>MGESERSEAFGIPRDSPLSSGDAAELEQLRREAAVLREQLENAVGSHAPTRSARDIHQLEARIDSLAARNSKLMETLKEARQQLLALREEVDRLGQPPSGYGVLLATHDDDTVDVFTSGRKMRLTCSPNIDAASLKKGQTVRLNEALTVVEAGTFEAVGEISTLREILADGHRALVVGHADEERVVWLADPLIAEDLPDGLPEALNDDTRPRKLRPGDSLLVDTKAGYAFERIPKAEVEDLVLEEVPDVSYADIGGLSRQIEQIRDAVELPFLHKELYREYSLRPPKGVLLYGPPGCGKTLIAKAVANSLAKKMAEVRGDDAHEAKSYFLNIKGPELLNKFVG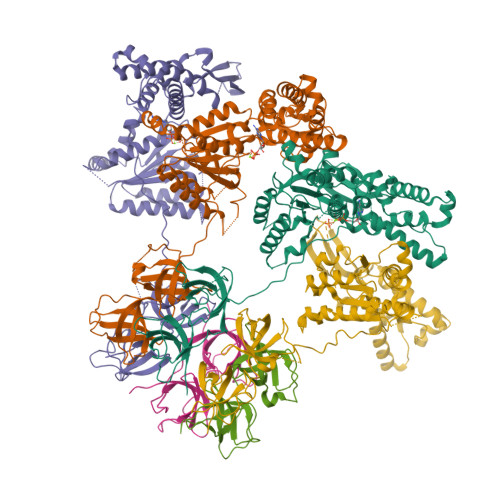ETERHIRLIFQRAREKASEGTPVIVFFDEMDSIFRTRGTGVSSDVETTVVPQLLSEIDGVEGLENVIVIGASNREDMIDPAILRPGRLDVKIKIERPDAEAAQDIYSKYLTEFLPVHADDLAEFDGDRSACIKAMIEKVVDRMYAEIDDNRFLEVTYANGDKEVMYFKDFNSGAMIQNVVDRAKKNAIKSVLETGQPGLRIQHLLDSIVDEFAENEDLPNTTNPDDWARISGKKGERIVYIRTLVTGKSSSASRAIDT[6x]2,4,5-trichlorophenol | C6 H3 Cl3 O | 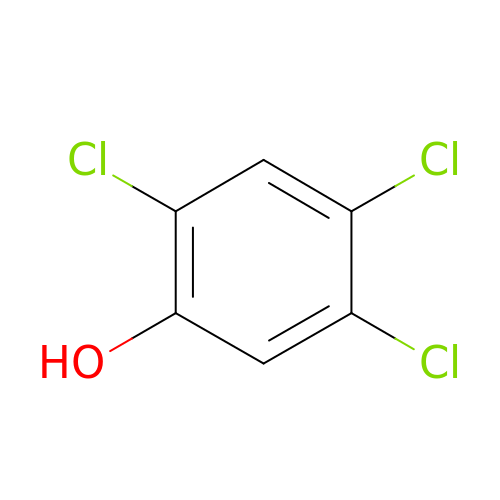LHJGJYXLEPZJPM-UHFFFAOYSA-N~{N}-[4-[4-[[4-(5-oxidanylidene-3-phenyl-6~{H}-1,6-naphthyridin-2-yl)phenyl]methyl]piperazin-1-yl]phenyl]propanamide | C34 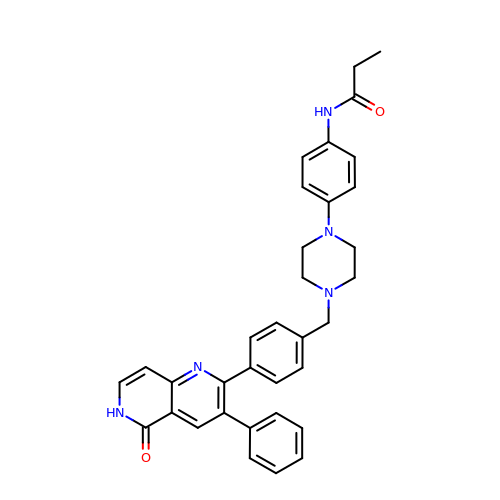H33 N5 O2 | QCTYKYAJKIOMDJ-UHFFFAOYSA-N>GSHMASQKTIRKIISSPLCPKPVGP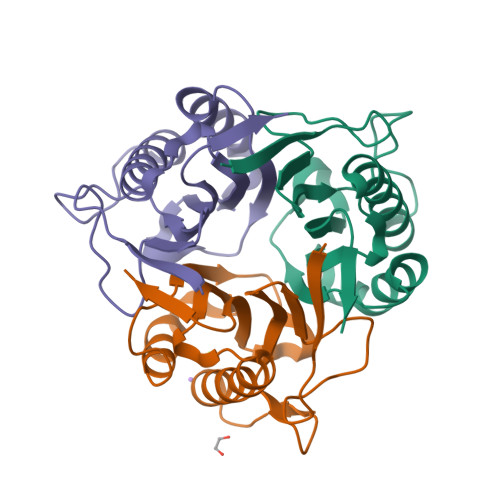YNQAILVNHTLYLSGILGIDVKTEKLVNGGAVAETRQALLNMGHILKEAGSNYNKVIKTTIFLQDINDFTDVNEVYKEFFKENYPARSTFQVGKLPMAAQLEIEAIAITGEVETI[3x]> MVSPTKMIIRSPLKETDTNLKHNNGIAASTTAAGHLNVFSNDNNCNNNNTTESFPKKRSLERLELQQQQHLHEKKRARIERARSIEGAVQVSKGTGLKNVEPRVTPKELLEWQTNWKKIMKRDSRIYFDITDDVEMNTYNKSKMDKRRDLLKRGFLTLGAQITQFFDTTVTIVITRRSVENIYLLKDTDILSRAKKNYMKVWSYEKAARFLKNLDVDLDHLSKTKSASLAAPTLSNLLHNEKLYGPTDRDPRTKRDDIHYFKYPHVYLYDLWQTWAPIITLEWKPQELTNLDELPYPILKIGSFGRCPFIGDRNYDESSYKRVVKRYSRDKANKKYALQLRALFQYHADTLLNTSSVNDQTKNLIFIPHTCNDSTKSFKKWMQEKAKNFEKTELKKTDDSAVQDVRNEHADQTDEKNSILLNETETKEPPLKEEKENKQSIAEESNKYPQRKELAATPKLNHPVLATFARQETEEVP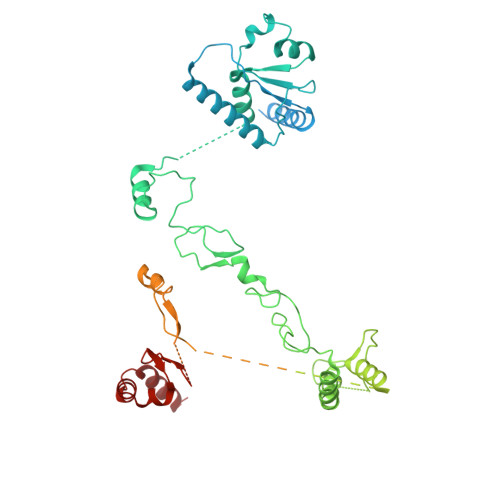DDLCTLKTKSRQAFEIKASGAHQSNDVATSFGNGLGPTRASVMSKNMKSLSRLMVDRKLGVKQTNGNNKNYTATIATTAETSKENRHRLDFNALKKDEAPSKETGKDSAVHLETNRKPQNFPKVATKSVSADSKVHNDIKITTTESPTASKKSTSTNVTLHFNAQTAQTAQPVKKETVKNSGYCENCRVKYESLEQHIVSEKHLSFAENDLNFEAIDSLIENLRFQI>[2x]EFSEDCENIFHDNAYLLKLDCEAGRVDPV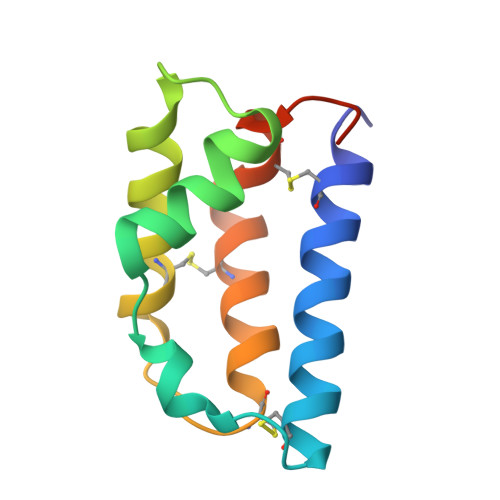EYDDISDEEIYEITVDVGVSSEDQEKVAKIIRECIAQVSTQDCTKFSEIYDCYMKKKICNYYPENMHHHHHH>MSDLDTPTPSPHPVLLNLEQFLPYRLSVLSNRISGNIAKVYGDRYGMAIPEWRVITILALYPGSSASEVSDRTAMDKVAVSRAVARLLERGFIRRETHGDDRRRSMLALSPAGRQVYETVAPLVNEMEQRLMSVFSAEEQQTLERLIDRLAKDG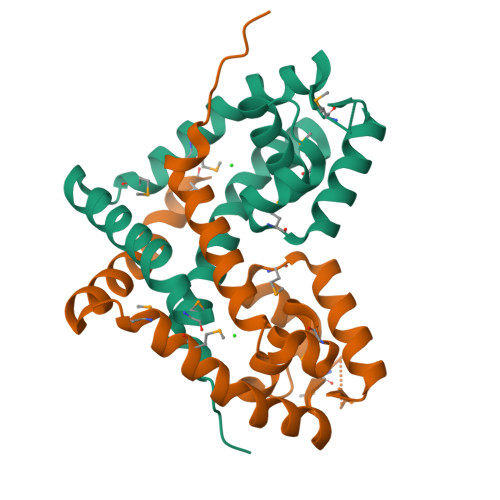LPRMASKD[2x]>MELFDENYYAKAVANIIGEVKDPIMYKWFSPDQIEDVDLQMGYQKTVKWDAFLNANPTTIANEVNTISTIGFSSEVVRLNYLKLQYKFRHLKQTSEKFYTSDSYIGDINNNLLPFAQAYKLASSEIIKLINHFVLTGTVSIQKDGKNQKRLLPNMYGLLNMPEQIKEEVASGDKDKMDKIFEKIEAGLSKLELGDEFSTPMMVIVDPATSLKLVKPYAAAQGAASSCEKWEDVLIQTIKAINNREDVYIETSNLLKHKILIYPLNSELIKFKPSKYMLPTPNEQVDKDSTDVAHSYIDFVLGGLLATRKTILQVNIKQS[27x];>[17x]MSDITKIKQEFDKKVAEIQALMKNPQQDSGLLSNSIDFRDQNLIFSNSGGVCTSSKDKIENYPAKGYPYKRGVKLSFGDGTTELEVEAGGGDDLYGVCSDIDEFSGMATVIPITNNFTGYLTLKKDGQNGVNPGDKLNFNQHGELEKVTGAQKSVNAIALSKAHKLTEDLFIVLASVFGNRAIKG;>MTEKEEKEDLQAQDKEEQQIKADTKVISVQEFEEYMRFKEQANSKSKETSRDLSINERITK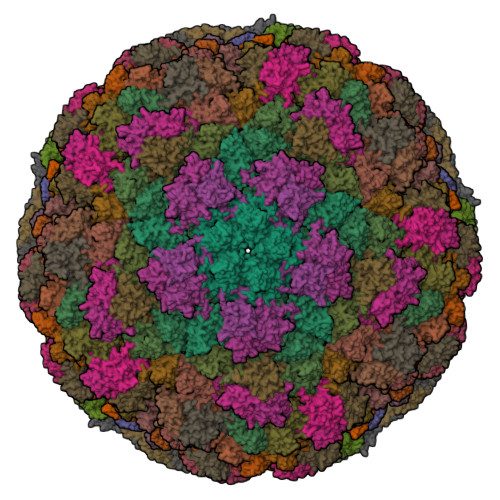ELAEVEERERIEKQLLLEAERINEIDTLAKAHLSNHFNKEVLLAKGYTLKDIMQAQRRELVRKFVPIEQIKAIAKVSDISHIDGEILEQLVSLAKVNIKLRKNASSSSSSVDSIKGNIAIKSEERASLLDSNFVPINFTEFVQAISNTYKQRRIQFYENLKRHKRTSIA[27x];>MGDTTQLVKEYQEKRSKLEKFMKNPQHDASLLSNSNEFRDKNVEFFASGGTRTSKFDKLENHPFLGYPYKRGVKRVIQEAQDNQSHYEPHVEAGGGEDLYGICIDIDEFSKTATIVPITNNFEGYLVAKDSTVKVKDKLIFNKDGALEKVTGAPNKATINATALTDAKQISNEVYLVKVAVFGNKAMSRN[7x]> MASGLYLFVMNIRSVFKLDELGSEVLRIAVPASLALAADPLASLVDTAFIGHLGSVEIAAVGVSIAIFNQVSKVCIYPLVSVTTSFVAEEDAIISKYLEEKKRYIPSVTSALIVGSFLGLVQAVFLIFSAKFVLGIMGVKHDSPMLEPAVRYLTIRSLGAPAVLLSLAMQGVFRGFKDTKTPLYATVVGDATNIILDPILMFVCHMGVTGAAVAHVISQYLITMILICRLVQQVDVIPPSLKSLKFGRFLGAGFLLLARVVAVTFCVTLASSLAARDGPTIMAAFQICLQLWLATSLLADGLAVAGQAVLASAFAKNDHKKVIAATSRVLQLSIVLGMGLTVVLGLFMKFGAGVFTSDADVINVIHKGIPFVAGTQTINALAFVFDGINFGAQDYVYSAYSMVGVASISIPCLVYLSAHKGFIGIWVALTIYMSLRTVASTWRMGAARGPWVFLRKAGGENLYFQ

HvAACT1, belonging to the MATE family, transports citrate from the root cells to the rhizosphere, where it chelates toxic Al ions externally, thereby conferring plants’ Al tolerance. While most structurally characterized MATE proteins transport cationic or aromatic substrates, HvAACT1 is unique in transporting anionic substrates. In general, MATE transporters share a common topology consisting of 12 transmembrane helices (TM), which form quasisymmetric lobes: the N-lobe (TM1-TM6) and the C-lobe (TM7-TM12). Our structure-based mutagenesis work identifies the citrate recognition and proton binding sites in HvAACT1, which are physically separated but functionally conjugated.

Here, we present the crystal structure of HvAACT1, a citrate MATE transporter from barley (Hordeum vulgare), in its outward-facing conformation at 3.2 Å resolution. Removing these regions (Δ1-56, Δ153-199) and introducing five-point mutations—C351A, C388L, T495V to enhance thermostability, along with R105H, R456S to reduce surface entropy—successfully enabled crystallization of a modified construct, hereinafter referred to as HvAACT1cryst. Functional assays in Xenopus oocytes confirmed that HvAACT1cryst retains citrate efflux activity comparable to the wild type, suggesting that the truncated N-terminal and L2-3 loop regions are not essential for citrate transport. The crystal structure of HvAACT1cryst adopts a typical V-shaped outward-facing conformation, similar to the previously reported MATE transporters. The twelve transmembrane helices of HvAACT1cryst form two distinct lobes: N-lobe (TM1-TM6) and C-lobe (TM7-TM12). These lobes make tight contacts on the intracellular side, sealing the transporter’s internal cavity from the cytoplasm for approximately 15 Å. The electrostatic surface potential of the inner cavity in HvAACT1cryst reveals a positively charged C-lobe, attributed to three basic residues: K126TM2, R358TM7, and R535TM12. Conversely, the N-lobe cavity is primarily negatively charged, owning to a cluster of four Asp residues (D92TM1, D99TM1, D289TM5, and D296TM5). Despite 0.1 M citrate in the crystallization buffer, no electron density corresponding to citrate was detected. In the HvAACT1cryst structure, D99TM1 forms a carboxyl–carboxylate interaction with D296TM5 at a distance of 2.7 Å, similar to the D41TM1/D184TM5 pair in PfMATE.> SPSAEACGYSDRVLQLKLGNSAIVTQEAANYCCAYGEWPNYLPDHEAVAIDKPTQPETATDRFYTLKSVKWETESTGWWWKLPDALNNIGMFGQNVQHHYLYRSGFLIHVQCNATKFHQGALLVVAI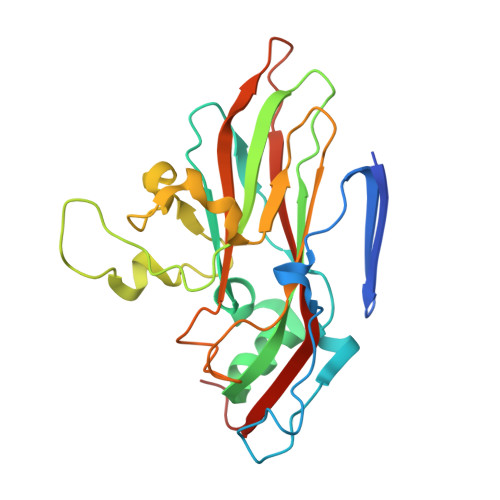PEHQRGAHNTTTSPGFDDIMKGEEGGTFNHPYVLDDGTSLACATIFPHQWINLRTNNSATIVLPWMNAAPMDFPLRHNQWTLAIIPVVPLGTRTVSSMVPITVSIAPMCCEFNGLRHAITQ>GSHMDNQCTVQVRLELGHRAQLRKKPTTEGFTHDWMVFVRGPEQCDIQ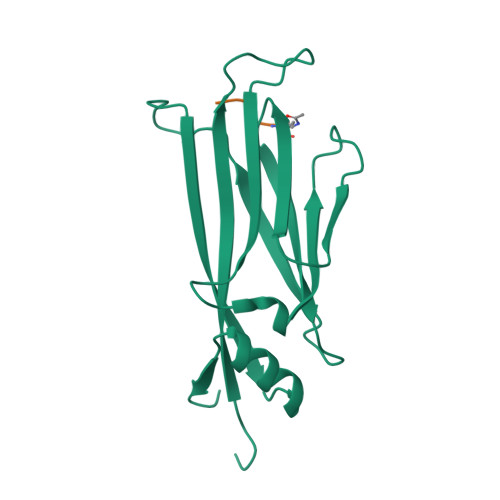HFVEKVVFWLHDSFPKPRRVCKEPPYKVEESGYAGFIMPIEVHFKNKEEPRKVCFTYDLFLNLEGNPPVNHLRHLRCEKLTFNNPTTEFRYKLLRAGGVMVMPEGAHHHHHH[2x];>[2x]AARK>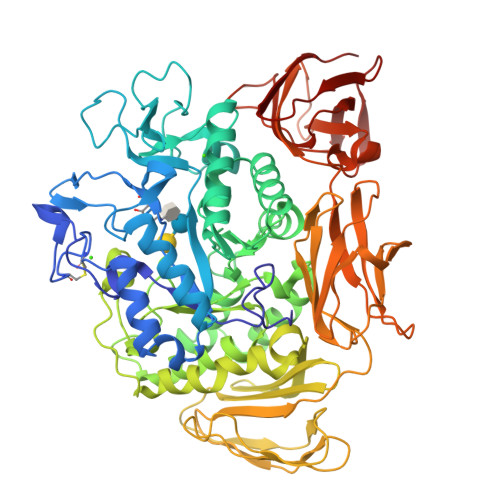[2x]APDTSVSNKQNFSTDVIYQIFTDRFSDGNPANNPTGAAFDGSCTNLRLYCGGDWQGIINKINDGYLTGMGITAIWISQPVENIYSVINYSGVNNTAYHGLWARDFKKTNPAYGTMQDFKNLIDTAHAHNIKVIIDFAPNHTSPASSDDPSFAENGRLYDNGNLLGGYTNDTQNLFHHYGGTDFSTIENGIYKNLYDLADLNHNNSSVDVYLKDAIKMWLDLGVDGIRVDAVKHMPFGWQKSFMATINNYKPVFTFGEWFLGVNEISPEYHQFANESGMSLLDFRFAQKARQVFRDNTDNMYGLKAMLEGSEVDYAQVNDQVTFIDNHDMERFHTSNGDRRKLEQALAFTLTSRGVPAIYYGSEQYMSGGNDPDNRARLPSFSTTTTAYQVIQKLAPLRKSNPAIAYGSTHERWINNDVIIYERKFGNNVAVVAINRNMNTPASITGLVTSLPRGSYNDVLGGILNGNTLTVGAGGAASNFTLAPGGTAVWQYTTDATTPIIGNVGPMMAKPGVTITIDGRGFGSGKGTVYFGTTAVTGADIVAWEDTQIQVKIPAVPGGIYDIRVANAAGAASNIYDNFEVLTGDQVTVRFVINNATTALGQNVFLTGNVSELGNWDPNNAIGPMYNQVVYQYPTWYYDVSVPAGQTIEFKFLKKQGSTVTWEGGANRTFTTPTSGTATVNVNWQP> MNYSYKRYWEPSTAEVIGLSLSVNTISAALTYPIEFVKVRSQIRTEGVGIRSKNLYMGINPNKVFREIHATGNGLRGFYQGFESHLIGRLSYLFIRNLTYKIIYDRTKPVKAHNDLSHREKGVIAGFAGGLAAFLTSPADLVNTRTIAEGGKPKEWRWGYKGLMDGINKIAATEGGNAALFRGSYANVLRAVILNISLTGPFDYLNEKI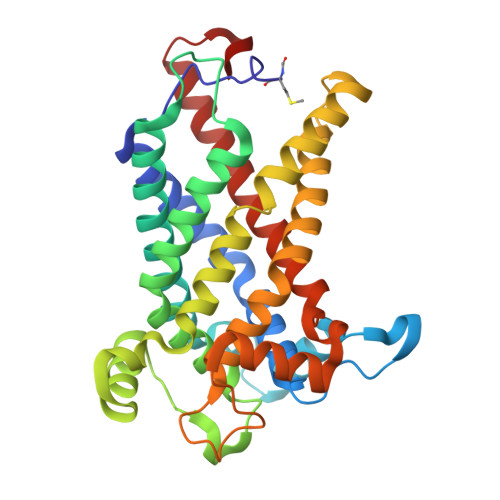WITFGDMTWNKYAALLWASFWGSVATLPFDNIRTRLYAQNADPTKNRLTYSGWADAAKKLIQHEGISGFYVGFYAFYIRTFLYAWTTVFITDKITSDWKRKAGLKEWQI>MGGHHHHHHGENLYFQGISSETGEMGILWEFDPIINKWIRLSMKLKVERKPFAEGALREAYHTVSLGVGTDENYPLGTTTKLFPPIEMISPISKNNEAMTQLKNGTKFVLKLYKKEAEQQASRELYFEDVKMQMVCRDWGNKFNQKKPPKKIEFLMSWVVELIDRSPSSNGQPILCSIEPLLVGEFKKNNSNYGAVLTNRSTPQAFSHFTYELSNKQMIVVDIQGVDDLYTDPQIHTPDGKGFGLGNLGKAGINKFITTHKCNAVCA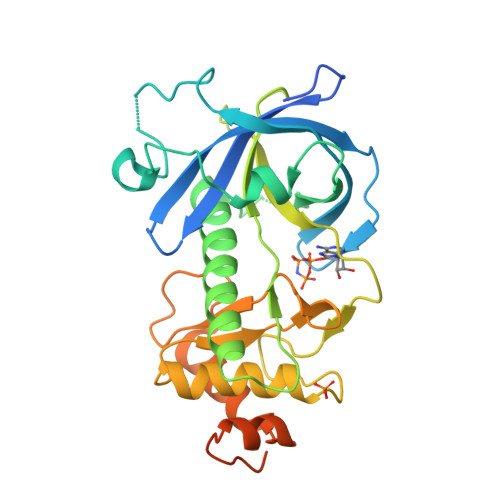LLDLDVKLGGVLSGNNKKQLQQGTMVMPDILPELMPSDNT[2x]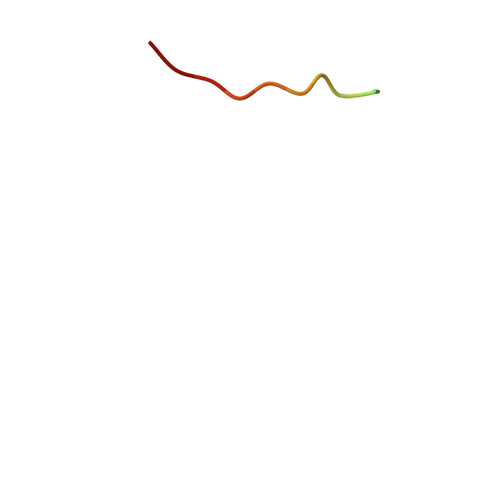> SPQGGGPWDSVARVL> MEPLYDKNGAVLFGEPSDTHPQSTLKLPHPRGEKEVIVGIRDLPRKGDCRTGNRLGPVSGLFVKPGP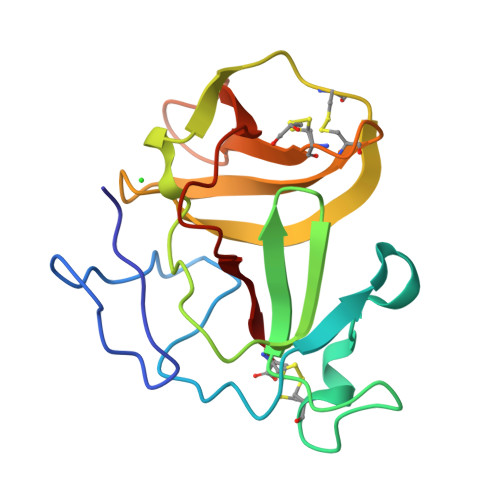VFYQDYSGPVYHRAPLEQFKQAPMCEVTKRIGRVTGSDGNLYHMYVCTDGCILVKTAKHHHHHVLKWVYNVLDSPIWVTSC(2R,4S)-2-[(1R)-2-butoxy-1-[(5-methyl-3-phenyl-1,2-oxazol-4-yl)carbonylamino]-2-oxidanylidene-ethyl]-5,5-dimethyl-1,3-thiazolidin-3-ium-4-carboxylic 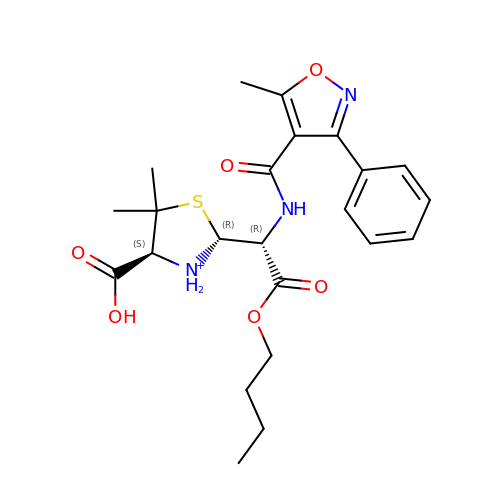acid | C23 H30 N3 O6 S | KTVAJMKGNMTGBA-CMKODMSKSA-O>[12x]SVIKPDMKIKLRMEGAVNGHPFAIEGVGLGKPFEGKQSMDLKVKEGGPLPFAYDILTT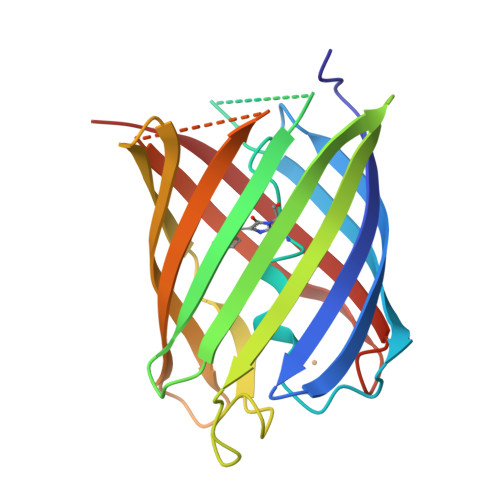VFSYGNRVFAKYPENIVDYFKQSFPEGYSWERSMNYEDGGICNATNDITLDGDCYIYEIRFDGVNFPANGPVMQKRTVKWEPSTEKLYVRDGVLKGDVNMALSLEGGGHYRCDFKTTYKAKKVVQLPDYHFVDHHIEIKSHDKDYSNVNLHEHAEAHSE> DKAMAGNFWQSSHYLQWILDKQDLLKERQKDLKFLSEEEYWKLQIFFTNVIQALGEHLKLRQQVIATATVYFKRFYARYSLKS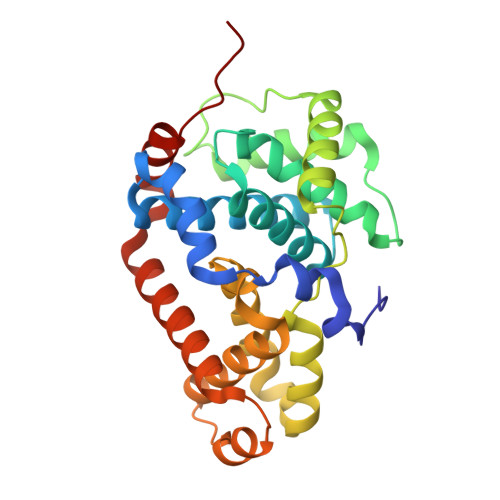IDPVLMAPTCVFLASKVEEFGVVSNTRLIAAATSVLKTRFSYAFPKEFPYRMNHILECEFYLLELMDCCLIVYHPYRPLLQYVQDMGQEDMLLPLAWRIVNDTYRTDLCLLYPPFMIALACLHVACVVQQKDARQWFAELSVDMEKILEIIRVILKLYEQWKNFDERKEMATILSKMPKPKPPP>[2x]GAMPHDPSFTPTQLAARAAYLLRGNDLGTMTTAAPLLYPHMWSWDAAFVAIGLAPLSVERAVVELDTLLSAQWRNGMIPHIVFANGVDGYFPGPARWATATLADNAPRNRLTSGITQPPVHAIAVQRILEHAR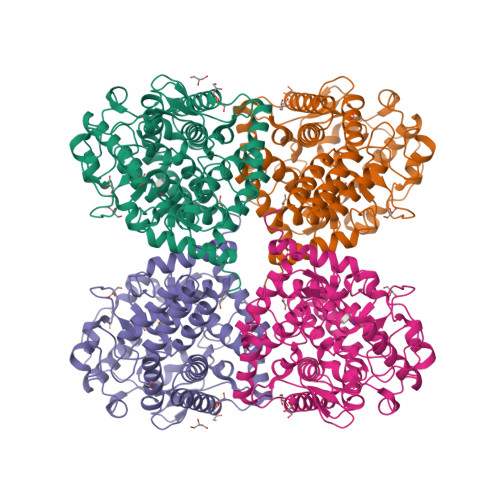TRGRSTRAVAEAFLDRRWGDLMRWHRWLAECRDRNERGRITLYHGWESGMANSPRWDSAYANVVPGKLPEYQRADNVIITDPSQRPSDGEYDRYLWLLEEMKAVRYDDERLPSVMSFQVEDVFFSAIFSVACQVLAEIGEDYKRPHADVKDLYLWAERFRAGVVETTDQRTGAARDFDVLAEKWLVTETAAQFAPLLCGGLPHDRERALLKLLEGPRFCGHPDLKYGLIPSTSPVSRDFRPREYWRGPVWPVLTWLFSWCFARRGWAERARLLRQEGLRQASDGSFAEYYEPFTGEPLGSMQQSWTAAAVLDWLG>[2x]MGSSHHHHHHSQASIFVDTSFWAALGNAGDARHGTAKRLWASKPPVVMTSNHVLGETWTLLNRRCGHRAAVAAAAIRLSTVVRVEHVTADLEEQAWEWLVRHDEREYSFVDATSFAV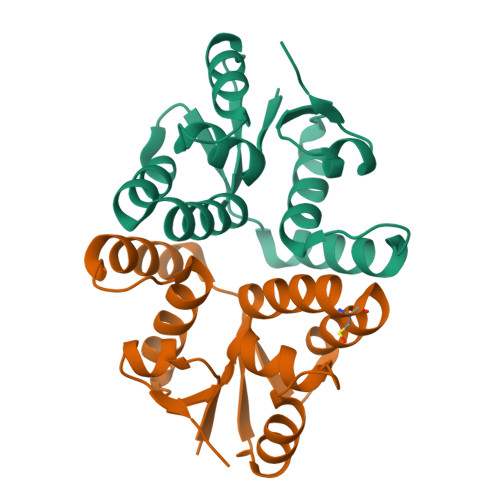MRKKGIQNAYAFDGDFSAAGFVEVRPE>MGSSHHHHHHSQDPMLSVGATTTATRLTGWGRTAPSVANVLRTPDAEMIVKAVARVAESGGGRGAIARGLGRSYGDNAQNGGGLVIDMTPLNTIHSIDADTKLVDIDAGVNLDQLMKAALPFGLWVPVLPGTRQVTVGGAIACDIHGKNHHSAGSFGNHVRSMDLLTADGEIRHLTPTGEDAELFWATVGGNGLTGIIMRATIEMTPTSTAYFIADGDVTASLDETIALHSDGSEARYTYSSAWFDAISAPPKLGRAAVSRGRLATVEQLPAKLRSEPLKFDAPQLLTLPDVFPNGLANKYTFGPIGELWYRKSGTYRGKVQNLTQFYHPLDMFGEWNRAYGPAGFLQYQFVIPTEAVDEFKKIIGVIQASGHYSFLNVFKLFGPRNQAPLSFPIPGWNICVDFPIKDGLGKFVSELDRRVLEFGGRLYTAKDSRTTAETFHAMYPRVDEWISVRRKVDPLRVFAS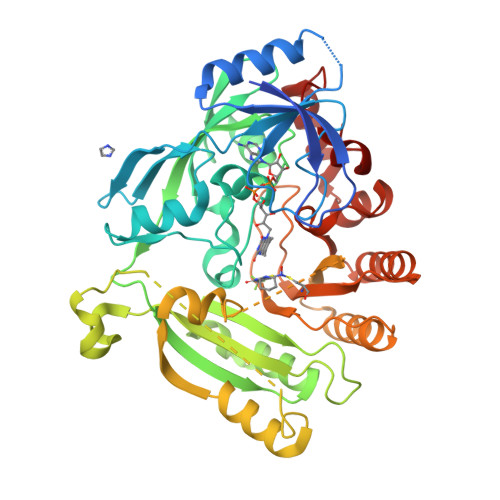DMARRLELL[2x]> MSEPTYFMPPEWAPHASTWLSWPHKLESWPGKFEPVPAVFAELAYQLSRSETVNINVLDDAMEAQARELLKERDPEGKYAERIVFHRIPTNDAWCRDHGPNYVIRTQDGRRDKVIMNWEYNAWGGKYEPYDDDNAVPERVAKAQGLPMVSTGMVLEGGAIDVNGAGLLLTTTACLLNPNRNPSLGKAEIEAQLRRYLGIEKVLWLGDGIAGDDTDGHVDDMARFVNENTVVIAVEEDPEDENYKPLRENYELLKTMTGLDGKPLNIVKLPMPEPVYYDGERLPASYANFYIANTVVLVPTYRCPRDQQAIDILQQCFP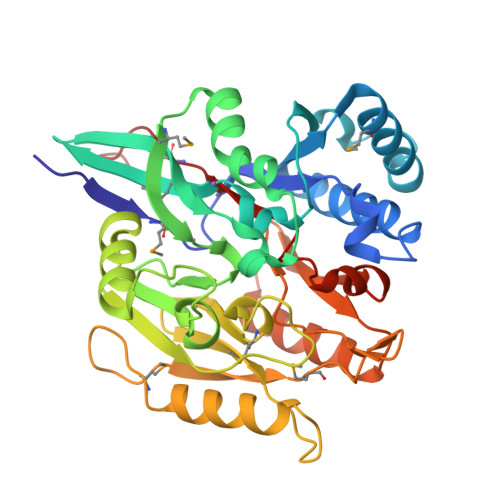KREVVGIDCSDLIWGLGAIHCVTHEEPAMLEHHHHHH>AAPPAPPVSYGVEEDVFHPVRAKQGMVASVDATATQVGVDILKEGGNAVDAAVAVGYALAVTHPQAGNLGGGGFMLIRSKNGNTTAIDFREMAPAKATRDMFLDDQGNPDSKKSLTSHLASGTPGTVAGFSLALDKYGTMPLNKVVQPAFKLARDGFIVNDALADDLKTYGSEVLPNHENSKAIFWKEGEPLKKGDTLVQANLAKSLEMIAENGPDEFYKGTIAEQIAQEMQKNGGLITKEDLAAYKAVERTPISGDYRGYQVYSMPPPSSGGIHIVQILNILENFDMKKYGFGSADAMQIMAEAEKYAYADRSEYL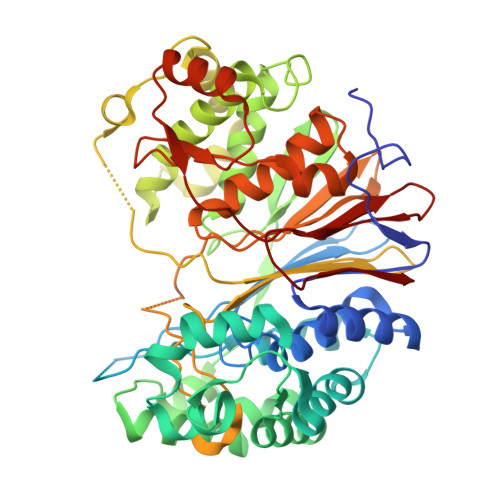GDPDFVKVPWQALTNKAYAKSIADQIDINKAKPSSEIRPGKLAPYESNQATHYSVVDKDGNAVAVTYTLNTTFGTGIVAGESGILLNNQMDDFSAKPGVPNVYGLVGGDANAVGPNKRPLSSMSPTIVVKDGKTWLVTGSPGGSRIITTVLQMVVNSIDYGLNVAEATNAPRFHHQWLPDELRVEKGFSPDTLKLLEAKGQKVALKEAMGSTQSIMVGPDGELYGASDPRSVDDLTAGY[2x]Apoptosis‐inducing protein of 56 kDa (AIP56) is a major virulence factor of Photobacterium damselae subsp. piscicida (Phdp), a Gram-negative bacterium that infects warm water marine fish with high economic importance for aquaculture. AIP56 is a short-trip single-chain AB toxin18,19 secreted by the type II secretion system of Phdp20. It has zinc-metalloprotease activity towards NF-kB p65, and targets fish phagocytes leading to their elimination by post-apoptotic secondary necrosis. In this work, the determination of the three-dimensional structure of AIP56 shows that, instead of a two-domain organization suggested by previous studies, AIP56 has three-domains: a non-LEE encoded effector C (NleC)-like catalytic domain associated with a small middle domain that contains the linker-peptide, followed by the receptor-binding domain.

The final crystallographic model of AIP56 does not include residues 290-295 (ND1), 362-385 (ND2), 422-429 (ND3) and 454–455 (ND4), which are poorly defined in the electron density maps. The three-dimensional structure of AIP56 shows a three-domain organization: (i) a N-terminal NleC-like catalytic domain (N1-F255) with a conserved zinc-binding motif (H165ExxH); (ii) a middle domain (G256-E307), with a disulfide bond (C262 and C298) flanking the 35 amino acid long linker peptide (S263 to E297), packed against the catalytic domain; and (iii) a C-terminal domain (P308-N497) previously shown to be involved in receptor binding. The active-site zinc ion of AIP56 is coordinated by H165 and H169 from helix α6 and by D176 located at the loop between helices α6 and α7. In two of the AIP56 monomers of the asymmetric unit, Y207 from the loop between helices α7 and α8 is the fourth zinc ligand, similar to what is observed in NleC24. The middle domain of AIP56 is composed of one α-helix (α10), two 310 helices (η5 and η6) and two short antiparallel β-strands (β4-β5). Two cysteine residues, one in helix α10 and the other in strand β5, form a disulfide bond previously shown to be important for AIP56 toxicity. These two cysteines flank the partially structured linker peptide that comprises helix η5 and strand β4 plus a connecting 15 residue-long unstructured loop (P270-A285) that contains an aspartate-rich patch at its tip (D274HDDD278). Although this domain shows some flexibility with respect to the catalytic and middle domains, it establishes a series of contacts with helix α2 of the catalytic domain that prevent large structural movements. At the C-terminal end of the catalytic domain of AIP56, a helical hairpin formed by two amphipathic helices (α8: D209 to H231 and α9: E234 to K247) contains residues potentially available for protonation (E214, E218, H222, H231 and E234).

>[4x]MTAIFSLAINSNFVLANNDKPDASDDKYADYVVRLGSEHPLNHTQIIELSSAVSRAVLLSYPNIIDRYTAAATEYTVIDALFHSPTFRHIVSFGLHNQQENLGHIRYTNEYEINNNREDEFSLVSEVSYDDIKSSNAQQVPLVAFYEAREDRATGTPIVNMGVAPSLFSGRYSWWQEALIHEIVHHVTGSSDTHEENKQGPTEILAQMVAAELHWAIPTFKGYSDPARVEAIQERDFHSLLNMFQRHGSELGFLFTRLATIAKGKKASPDFGTLTSFCSEGISSFPKYPDHDDDFNGGGAFFLPSASADSSVECTFDVLNRIEPVDDSIKFEGGNLLIKNDFKNLNLRVAQLSFLNAKKGSGFYRKNWDSWKSWYQASSWKNGLNSGLYGYGHDESEGNLIYSPYGITFNDGSFSIGFSSRKHINDNTKDDNFVKLNNANWSSFYYAGQMFFDKNKRPVALVITEPLNAAFGAGWSYIYKDGKWHYEAQDDWDQRLFKDSTLSLDPHAPQFINLEHHHHHH>[4x]MGHSALMKGTLTLKGIPGGAECSVDIQGNDQMQFNTNAITVDKSCKQFTVNLS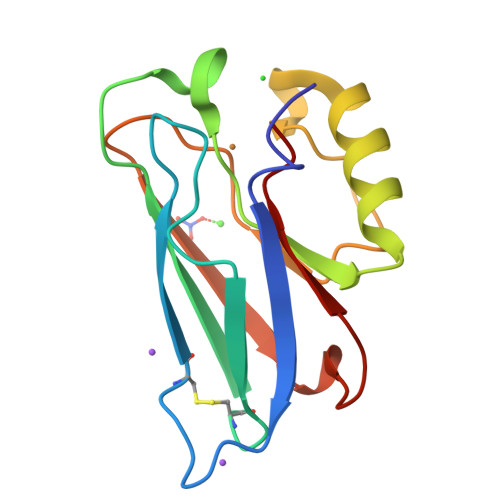HPGNLPKNVMGHNWVLSTAADMQGVVTDGMASGLDKDYLKPDDSRVIAHTKLIGSGEKDSVTFDVSKLKEGEQYMFFCTF> MVENNYLSVSEKTELEIAKQKLKNSKDPAEREKAQQKYDALLE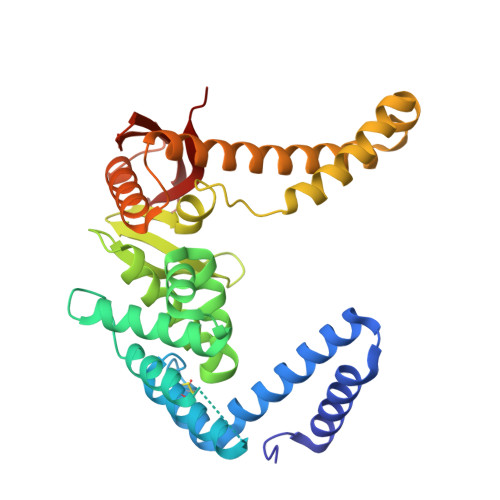KDISSDKAVITACSNGQAASAACAGERLKVIAAKGGYETGHYNNQVSDMYPDAYGQIVNLLNITSVDAQNQQQVKDAMVNYAMVQFGVDRATAQAYVETYDGMKVVAASMAPVIGAAAASKIEVLAGKQRLSNSFEVSSLPDANGKNHITAVKGDAKIPVDKIELYMRGKASGDLDSLQAEYNSLKDARISSQKEFAKDPNNAKRMEVLEKQIHNIERSQDMARVLEQAGIVNTASNNSMIMDKLLDSAQGATSANRKTSVVVSGPNGNVRIYATWTILPDGTKRLSTVNTGTFK chrysin | C15 H10 O4 | 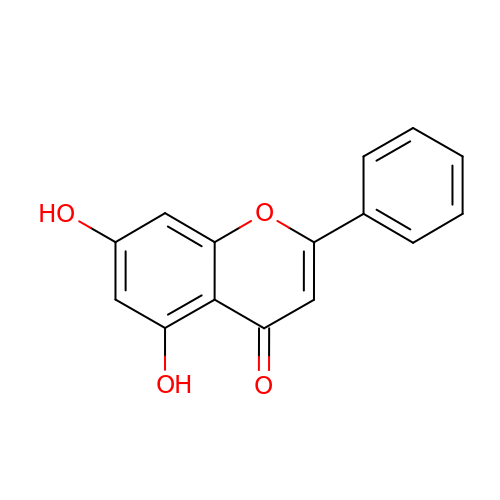RTIXKCRFFJGDFG-UHFFFAOYSA-N4-{[(E)-2-(5-CHLOROTHIEN-2-YL)VINYL]SULFONYL}-1-(1H-PYRROLO[3,2-C]PYRIDIN-2-YLMETHYL)PIPERAZIN-2-ONE 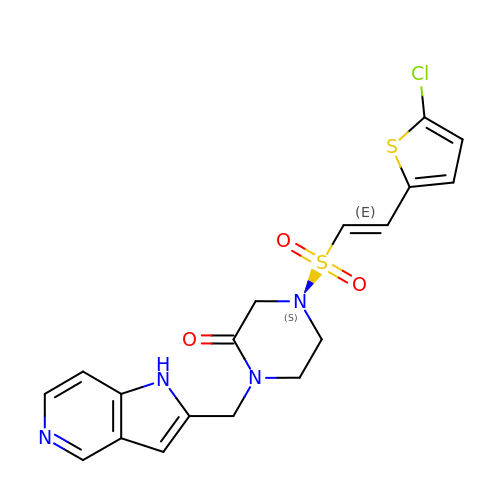| C18 H17 Cl N4 O3 S2 | PLWVUIRWJVKSSD-XBXARRHUSA-N> GVALGATRVIYPAGQKQEQLAVTNNDENSTYLIQSWVENADGVKDGRFIVTPPLFAMKGKKENTLRILDATNNQLPQDRESLFWMNVKAIPSMDKSKLTENTLQLAIISRIKLYYRPAKLALPPDQAAEKLRFRRSANSLTLINPTPYYLTVTELNAGTRVLENALVPPMGESTVKLPSDAGSNITYRTINDYGALTPKMTGVME;> DLYFNPRFLADDPQAVADLSRFENGQELPPGTYRVDIYLNNGYMATRDVTFNTGDSEQGIVPCLTR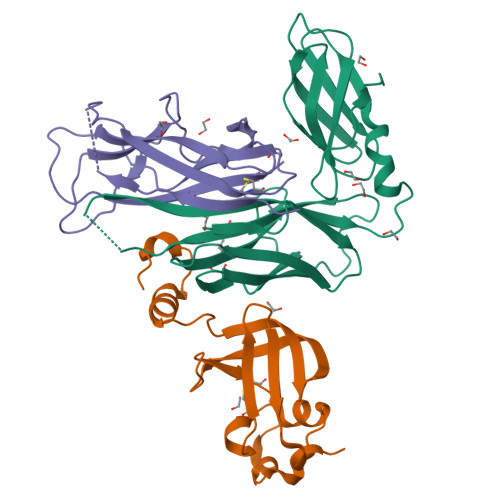AQLASMGLNTASVAGMNLLADDACVPLTTMVQDATAHLDVGQQRLNLTIPQAFMSNRAR;> DNGCSVAAESTNFTVDLMENAAKQFNNIGATTPVVPFRILLSPCGNAVSAVKVGFTGVADSHNANLLALENTVSAASGLGIQLLNEQQNQIPLNAPSSALSWTTLTPGKPNTLNFYARLMATQVPVTAGHINATATFTLEYQ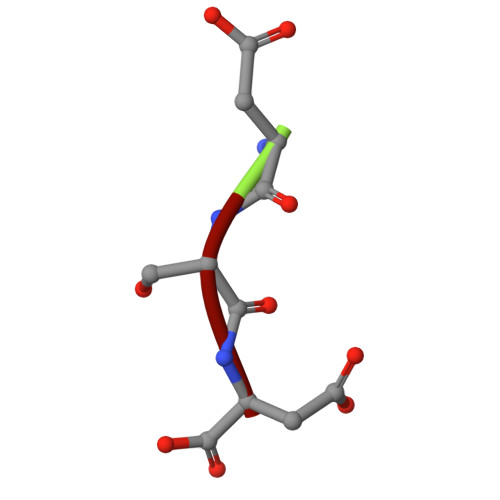> DSD>APLAATASKFLGCAYGAQQAPGFAQYWNKLTPENGGKWGSVEAVRDQMDWSTLDAAYRFAQANQMPFQMHVMVWGNQQPEWIKTLRPAEQRREIEQWFAAVAQRYPDIALLEVVNEPLNDPPSKADTGGGNYLQALGGNGDSGWEWVLQSFRLARRHFPHTKLMINDYSITSSAQATQKYLQIVRLLQRENLVDAIGVQEHAFETTPEVAVSVHRDNLDALAATGLPIYITEFDLDGPTDAQQLADYKRVFPVFWEHPAVHGITLWGFRPGLWRDKEAAYLIRADGTERPAL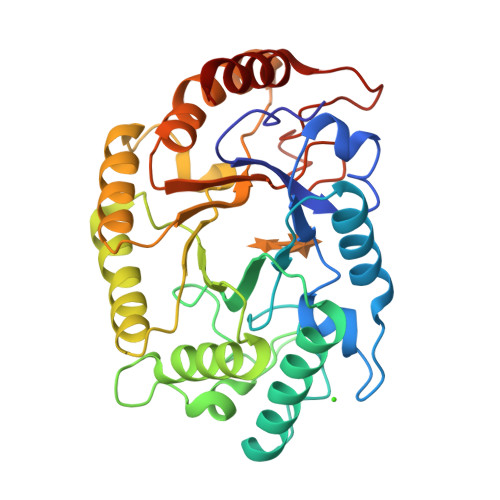TWLRDYVAAHP[2x]> QYKSI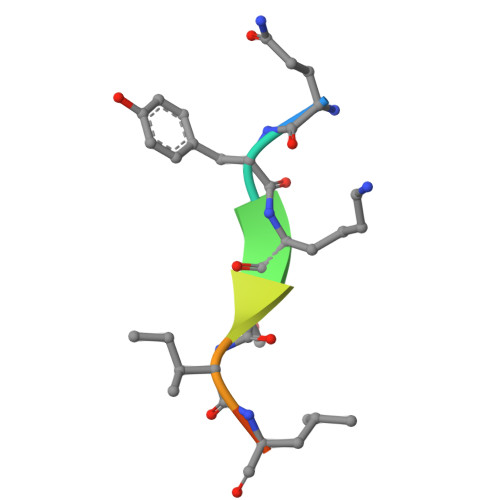LQE>MNLKDKILGVAKELFIKNGYNATTTGEIVKLSESSKGNLYYHFKTKENLFLEILNIQESKWQEQWKKEQIKAKTNREKFYLYNELSLTTEYYYPLQNAIIEFYTEYYKTNSINEKMNKLENKYIDAYHVIFKEGNLNGEWSINDVNAVSKIAAN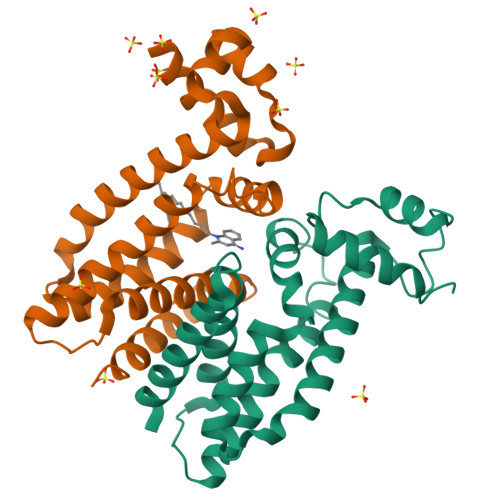AVNGIVTFTHEQNINERIKLMNKFSQIFLNGLSK[4x]> MAGDKGGGDGERRLRQPIVVVLGHVDHGKTTLLDKIRRTAVAAKEAGGITQHIGASIVPADVIEKIAEPLKKVIPVKLVIPGLLFIDTPGHELFSNLRRRGGSVA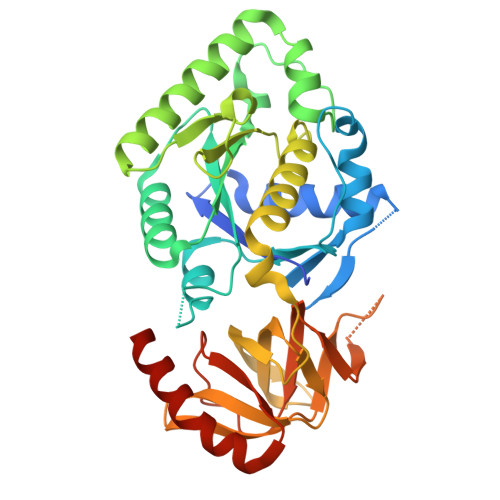DFAILVVDIMEGFKPQTYEALELLKERRVPFLIAANKIDRIPGWKPNPDAPFIETIRRQDPKVREILEQRVYEIVGKMYEAGLPAELFTRIKDFRRKIAIVPVSARTGEGIPELLAVLAGLTQTYLKERLRYAEGPAKGVVLEVKEMQGFGTVVDAVIYDGVLKKEDIIVVGGREGPIVTRVRALLMPAPLQDIRSREARFVQVDRVYAAAGVRIAAPGLDDVIAGSPIYAAESEEEARKLMEAVQREIEELRHHHHHH>GSAPSVKGVSFDQANNLLIEPARIEEEELTLTILRQTGGLGISIAGGKGSTPYKGDDEGIFISRVSEEGPAARAGVRVGDKLLEVN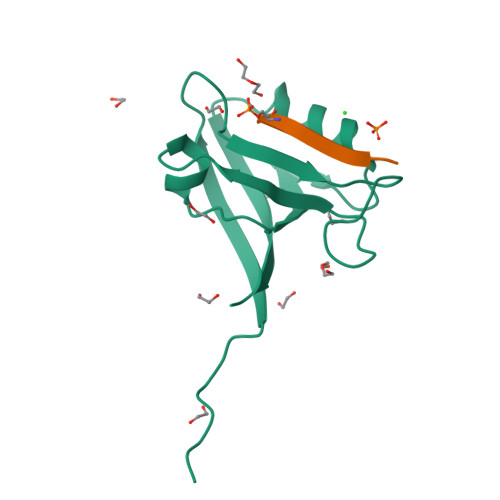GVALQGAEHHEAVEALRGAGTAVQMRVWRERM[2x];>PHTNETSL[2x]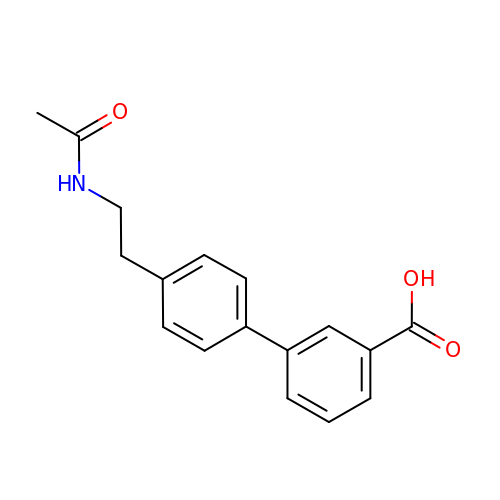3-[4-(2-acetamidoethyl)phenyl]benzoic acid | C17 H17 N O3 | OGVOCGQIMXHGHF-UHFFFAOYSA-N>HHHHHHMEKKLSDAQVALVAAWRKYPDLRESLEEAASILSLIVFQAETLSDQANELANYIRRQGLEEAEGACR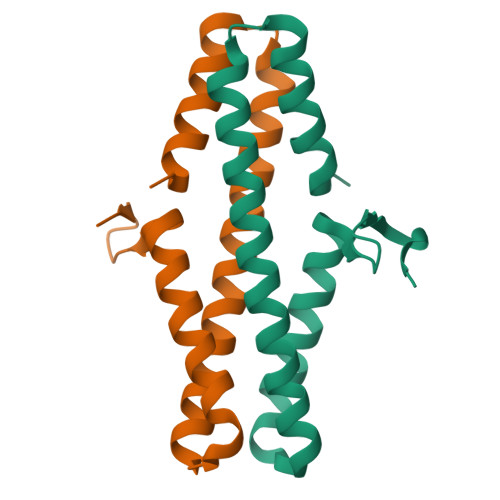NIDIMRAKWVEVCGEVNQYGIRVYGDAIDRDVD[4x]> 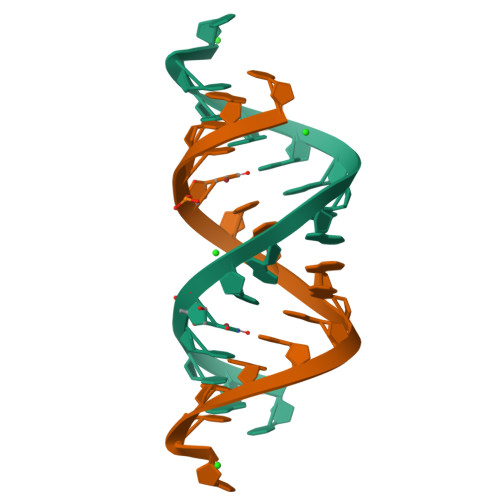CGCUUCGAAAAAGUC N-cycloheptyl-1-[(2,4,6-trimethylphenyl)sulfonyl]piperidine-4-carboxamide | C22 H34 N2 O3 S | 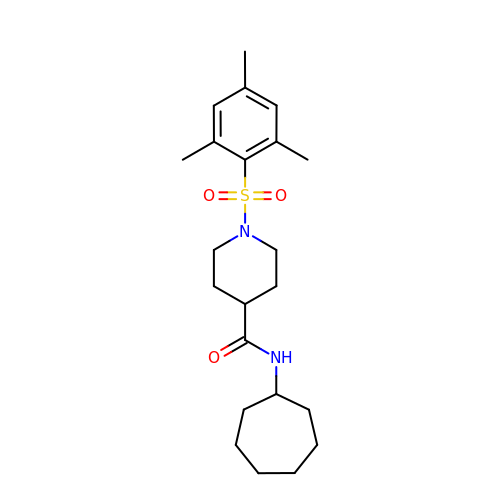GTZJATJFRQCZIY-UHFFFAOYSA-N> GDNQDRTVANTQPSGPSNSKEIPALTAVETGHTSQVDPSDTLQTRHVVNFHSRSESTVENFMGRAACVFMDQYKLNGEETSTDNFAVWTINVREMAQLRRKCELFTYMRFDIEMTMVITSCQDQGTQLEQDMPVLTHQIMYVPPGGPIPAKVDSY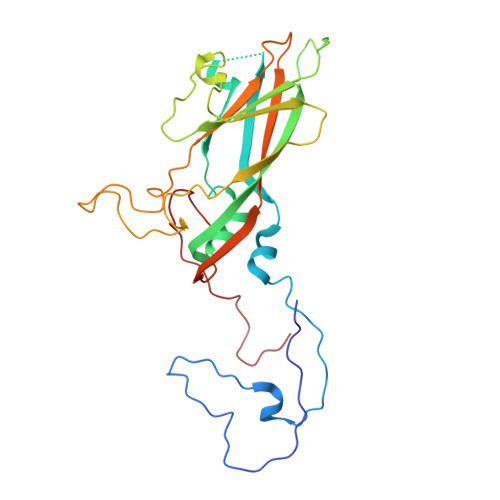EWQTSTNPSVFWTEGNAPARMSIPFISVGNAYSLFYDGWSHFTQDGTYGYTTLNAMGKLFVRHVNKSSPHQITSTIRVYFKPKHIKAWVPRPPRLCPYINKGDVNFVVTEVTDARKSITDTP> PAQDNSRFVIRDRNWHPKALTPDYKTSIARSPRQALVSIPQSISETTGPNFSHLGFGAHDHDLLLNFNNGGLPIGERIIVAGRVVDQYGKPVPNTLVEMWQ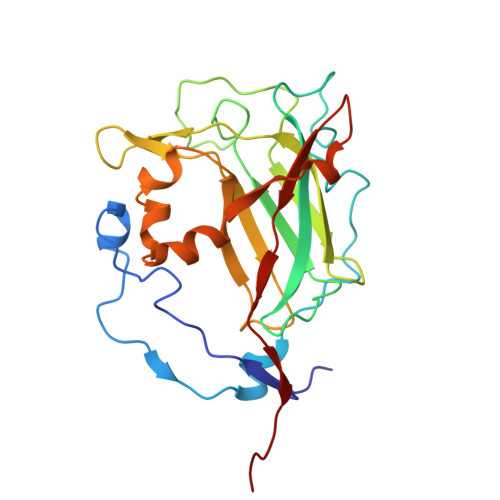ANAGGRYRHKNDRYLAPLDPNFGGVGRCLTDSDGYYSFRTIKPGPHPWRNGPNDWRPAHIYFGISGPSIATKLITQLYFEGDPLIPMCPIVKSIANPEAVQQLIAKLDMNNANPMDCLAYRFDIVLRGQRKTHFENC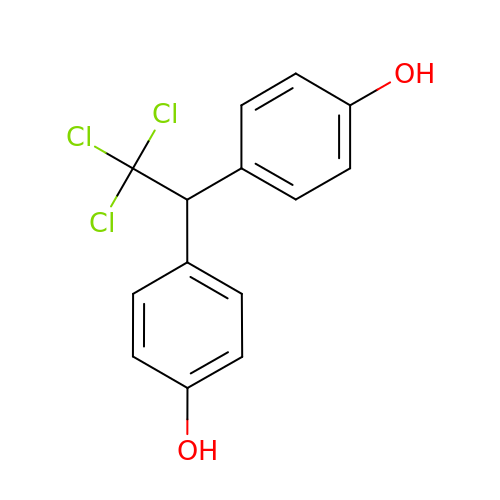4,4'-(2,2,2-trichloroethane-1,1-diyl)diphenol | C14 H11 Cl3 O2 | IUGDILGOLSSKNE-UHFFFAOYSA-N> QYDDHPPVFQKKFYIGGVSEDARMFASVLRVKATDRDTGNYSAMAYRLIIPPIKEGKEGFVVETYTGLIKTAMLFHNMRRSYFKFQVIATDDYGKGLSGKADVLVSVV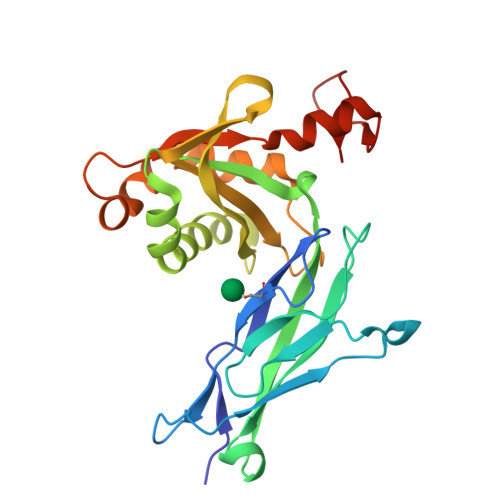NQLDMQVIVSNVPPTLVEKKIEDLTEILDRYVQEQIPGAKVVVESIGARRHGDAYSLEDYSKCDLTVYAIDPQTNRAIDRNELFKFLDGKLLDINKDFQPYYGEGGRILEIRTPEAVTSIKKRGESLGYTEGASRLVPR1-azanylpropylideneazanium | C3 H9 N2 | 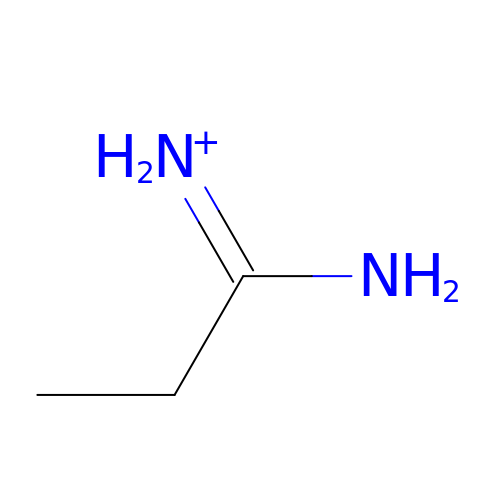GNFWGDKKNWGGJY-UHFFFAOYSA-O(1S,3R)-5-[4-(8-nitroquinolin-5-yl)piperazin-1-yl]carbonyladamantan-2-one 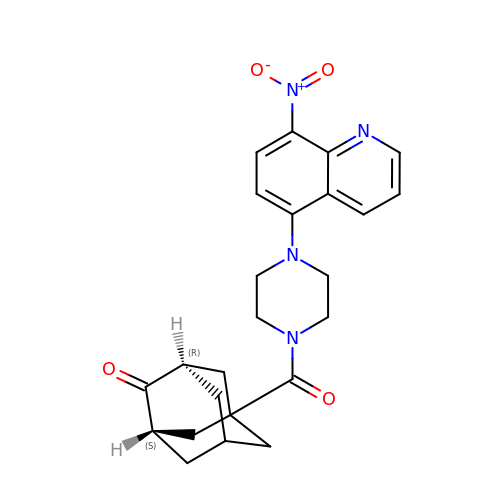| C24 H26 N4 O4 | RVHYZBKVITVCLB-XCEIDSMSSA-N>MKNFYDWIKEFIRDQGEFIAQQSGWLELERSSYAKLIAQTISHVLNGGSLLVSADSSRHWFLNYILSNLNPKDLKERPLLSVIDFNASSFYPKNDANLSLATIEMTYQNPMFWHVGKIENEGLKTILLSKIPSFLWLFEELKEDCLLLKEHDSLLDYKLLQLFKLFENALFSVLY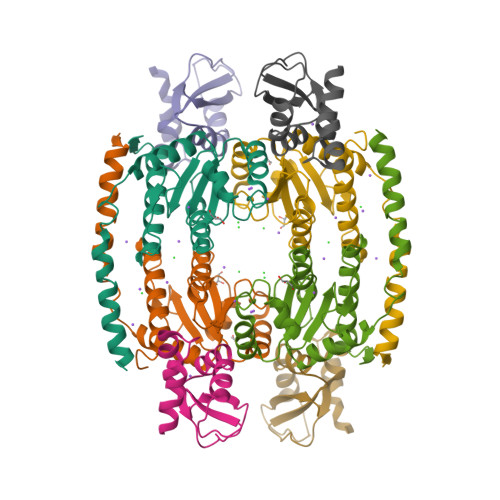NKVTL[2x];>MDTNNNIEKEILALVKQNPKVSLIEYENYFSQLKYNPNASKSDIAFFYAPNQVLCTTITAKYGALLKEILSQNKVGMHLAHSVDVRIEVAPKIQINAQSNINYKAIKTSVKD[2x]> KHLPEPFRIRVIEPVKRTTRAYREEAIIKSGMNPFLLDSEDVFIDLLTDSGTGAVTQSMQAAMMRGDEAYSGSRSYYALAESVKNIFGYQYTIPTHQGRGAEQIYIPVLIKKREQEKGLDRSKMVAFSNYFFDTTQGHSQINGCTVRNVYIKEAFDTGVRYDFKGNFDLEGLERGIEEVGPNNVPYIVATITSNSAGGQPVSLANLKAMYSIAKKYDIPVVMDSARFAENAYFIKQREAEYKDWTIEQITRETYKYADMLAMSAKKDAMVPMGGLLCMKDDSFFDVYTECRTLSVVQEGFPTYGGLEGGAMERLAVGLYDGMNLDWLAYRIAQVQYLVDGLEEIGVVCQQAGGHAAFVDAGKLLPHIPADQFPAQALACELYKVAGIRAVEIGSFLLGRDPKTGKQLPCPAELLRLTIPRATYT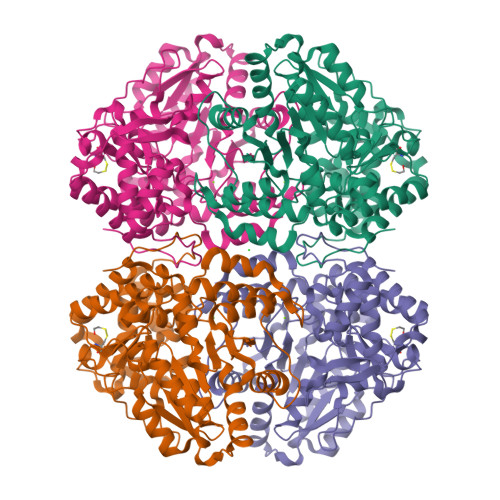QTHMDFIIEAFKHVKENAANIKGLTFTYEPKVLRHFTAKLKEV>MDLKTAVFNAARDGKLRLLTKLLASKSKEEVSSLISEKTNGATPLLMAARYGHLDMVEFLLEQCSASIEVGGSVNFDGETIEGAPPLWAASAAGHLKVVQSLLNHGASVNNTTLTNSTPLRAACFDGHLEIVKYLVEHKADLEVSNRHGHTCLMISCYKGHKEIAQYLLEKGADVNRKSVKGNTA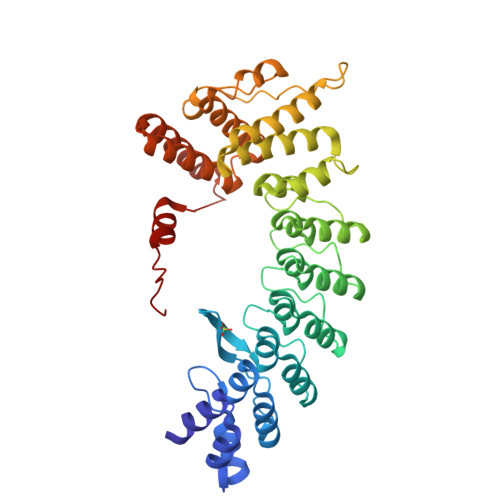LHDCAESGSLDIMKMLLMYCAKMEKDGYGMTPLLSASVTGHTNIVDFLTHHAQTSKTERINALELLGATFVDKKRDLLGALKYWKKAMNMRYSDRTNIISKPVPQTLIMAYDYAKEVNSAEELEGLIADPDEMRMQALLIRERILGPSHPDTSYYIRYRGAVYADSGNFKRCINLWKYALDMQQSNLDPLSPMTASSLLSFAELFSFMLQDRAKGLLG[2x]>RQRWTALT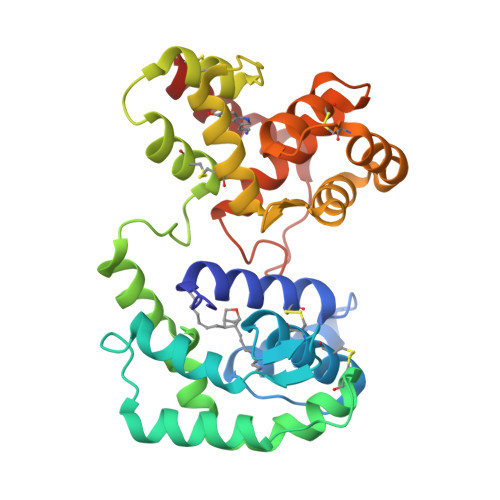PEETLFIYTRCQEEHLPADNNSRKTYIENWHQWKLQPNDHVTQCYTKCVLEGLELYDGKQKKFRPGRVSSQHVAYQFLNGATADEVAKYKGAIDALEPASDSCEDLYMAYFPVHETFVNVTRKLYHGTVEGAARVYNSDPNLKRKNESLFTYCEKHVYGDQNREDMCRGRRYELTGSDELRNMIECVFRGLRYIKHGDINIDEIVRDFDHINRGDLEPRVRTILSDCRGIQPYDYYSCLINSDIREEFKLAFDYRDVRSADYAYIVKGNTYDAQKVIAEMNKVEKHVCG[4x]>GAINLYSSRHYDTDQALYDSFTKKTGLKVNLIEGKGDKLIERIKSEGANSPADVFMTVDAGRLWRAQEAGILQPISSSTLNNKIPANLRSPEKLWFGFSKRARVIMYNKNKVQPSELSTYEDLAQNKWKGKIVIRSSSNIYNQSLIASLIEIHGMSDAEGWAKGFVRNFARPPEGNDTAQIKAVAAGIGDIGLANSYYLARLKRSSKPEDQAVADKVGMFFPNQNGRGTHVNISGGGVVKNAPNKEGAIKFLEYLVSPEAQKIFSEGNNEYPVVAGVPIASVLKPFGSFKNDSTNVSVYGKLNADAIKLMDRVGWKLE[2x]

We have investigated the function and structure of Trichodesmium Tery_3377, an iron stress-induced protein (iron deficiency-induced A, IdiA) commonly used as an in situ marker of iron stress. Using heterologous expression in the model cyanobacteria Synechocystis PCC6803, we provide evidence that Tery_3377, a commonly used iron-limitation biomarker, is localized to the periplasm with a suggested FutA2 function as an iron-binding protein of an ABC transporter. The overall fold of Tery_3377 assumes a classic small molecule ABC transporter substrate-binding domain fold, with two domains hinged over a substrate-binding cleft. The hinge region is formed by two short β-strands and connects the protein domains via a double cross-over between the N (residues 34–133 and 266–349) and C termini (134–265). This type of structure places Tery_3377 among class IV iron-binding proteins (in keeping with Ref. 27) and allows for structural classification within cluster D of the substrate-binding domains.

Amino acid additives in the crystallization buffers lead to the most ordered and best diffracting crystals. The best diffracting crystals were obtained with an additive mixture of amino acids. An amino acid ligand, alanine, is identified in the iron-binding cleft; the amino acid is ordered and coordinates the iron substrate. The geometry observed is trigonal bipyramidal, with the buffer molecule alanine carboxyl group, Tyr-174 and Tyr-231, forming the trigonal plane with angles of 108°, 108°, and 144°. Tyr-230 and the amino group from the buffer alanine coordinate the axial iron positions. The coordinating oxygen of the carboxylic acid moiety of the alanine ligand ideally superposes with a tyrosine side chain oxygen, whereas the amino nitrogen of the alanine ligand superimposes with a nitrogen from an interacting histidine ligand. The two coordinating amino-acids in FutA2 are contributed by a loop that is brought into the vicinity of the iron-binding site by domain closure around the hinge that brings the two lobes of the substrate-binding domain closer together. Interestingly, this motif is conserved in Tery_3377, and such a domain closure, although not observed under any of our crystallization conditions, can be proposed. We conclude that the alanine ligand mimics this iron-binding mode, leading to a pentacoordinated state. The observed binding of organic ligands together with iron may just be a fortuitous observation, but it might also have biological significance. It could be argued that the high concentrations of alanine present in crystallization mixtures out-competes interactions with the N-terminal iron-coordination residues His-43 and Tyr-44, thus leading to preferred crystallization of an open conformation.The Rex family members are well-conserved transcription factors to control the respiratory pathway, which senses changes in the redox state according to the intracellular NAD+/NADH balance. When the reduced NADH level is elevated, NADH is bound to a Rex protein, causing it to dissociate from the Rex DNA operator. TmRex forms a homodimer, and each monomer was composed of two distinct domains: the N-terminal domain involved in DNA binding and the C-terminal domain involved in NAD binding, which were linked by a flexible loop (residues 78–83). The last helix α9 of the C-terminal domain was mainly responsible for dimerization through the formation of a hydrophobic interface by extending to between the N- and C-terminal domains of the other subunit.

Subsequently, the native structure of apo TmRex was refined to 2.0 Å resolution with crystallographic Rwork and Rfree values of 20.40% and 25.83%, respectively. The refined model contained four TmRex subunits which formed two homodimers in an asymmetric unit. One dimer formed by subunits A and B was well ordered because of crystal contact stabilization, and the residues 4–208 in the subunit A and the residues 9–208 in the subunit B were interpretable. However, the N-terminal domains of the other dimer, formed by subunits C and D, were poorly ordered (average B-factors 79.6 Å2 and 73.1 Å2, respectively). Particularly, the glycine-rich loop comprising residues 55–63 was not visible due to the lack of electron-density maps. The initial structure of the apo TmRex was determined at 2.8 Å resolution using selenomethionine-based single-wavelength anomalous dispersion (SAD) data set collected at the selenium peak (0.9791 Å). The refined models of TmRex contained either two independent dimers (apo and NAD+-bound forms) or one dimer (NADH-bound form) in each asymmetric unit.

>MAEKIPKPVSKRLVSYYMCLERLLDEGVEVVSSEELARRLDLKASQIRKDLSYFGEFGKRGVGYNVEHLYDAIGEILGVKKEWKLVVVGAGNIGRAVANYTVMKEKGFRIIGIFDSDPSKIGKEAAPGLTVSDVSELEKFVEEHGVEIGVIAVPAEHAQEIAERLEKAGIKGILNFAPVKIKVSVPVENIDITASLRVLTFEIVRRNS[4x]>MGGVVGEALWQGGLEEALRAWLREDLGQGDLTSLLVVPEDLEGEAVILAKEGGVLAGLWVAERVFALADPRTAFTPLVAEGARVAEGTEVARVRGPLRGILAGERLALNLLQRLSGIATLTRAYVEALAGTKAQILDTRKTTPGLRALEKYAVRVGGGRNHRYGLFDGILLKENHVRAAGGVGEAVRRAKARAPHYLKVEVEVRSLEELEEALEAGADLILLDNFPLEALREAVRRVGGRVPLEASGNMTLERAKAAAEAGVDYVSVGALTHSAKALDLSLLV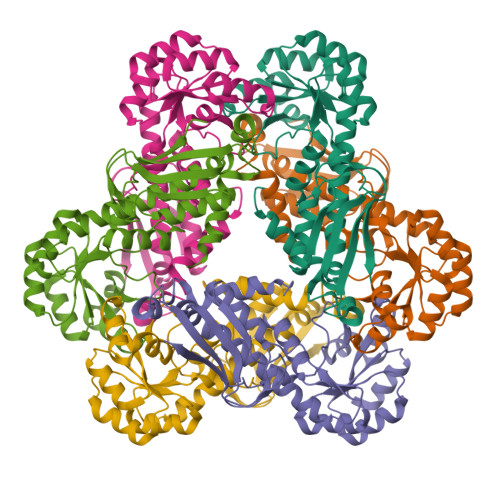VRP[3x]Transfer RNA–guanine transglycosylase (Tgt, EC 2.4.2.29) catalyses the exchange of a specific guanine base in tRNA molecules by a substituted 7-deazaguanine. Bacterial Tgt functions as a homodimer in which the protomer consists of a (βα)8 barrel harbouring a Zn2+ binding subdomain close to the C-terminus. The reaction follows a ping-pong mechanism including a covalent Tgt⋅tRNA intermediate. Hence, in an attempt to generate a model system for the active site of human Tgt and to gain insights into the relevance of particular amino acids for substrate base selectivity, we adapted the Z. mobilis Tgt active site by site-directed mutagenesis in order to mimic that of the human enzyme.

Comparison of the active centre of Z. mobilis Tgt with the modelled human Tgt catalytic subunit reveals that Ala232 adjacent to Val233 in the bacterial enzyme is replaced by a serine (Ser231) in human Tgt. As this residue is replaced by a serine in many bacterial Tgts too, it seems unlikely that it contributes to substrate specificity or catalytic activity. Nevertheless, we introduced the Ala232Ser mutation into Tgt(Cys158Val/Val233Gly) to investigate its impact. Kinetic measurements showed that the Ala232Ser conversion further reduced the catalytic activity of Tgt(Cys158Val/Ala232Ser/Val233Gly). Therefore, the Ala232Ser variants of Tgt were not considered further in this study. In addition, crystal structures that were determined of Tgt(Cys158Val/Ala232Ser/Val233Gly) in its apo-form, in complex with preQ1 and in complex with queuine do not show any significant differences to the corresponding ones of Tgt(Cys158Val/Val233Gly) and, due to redundance, will not be discussed in detail (data statistics and PDB codes of these structures are provided in Table S2 of the Supporting Information).

> VEATAQETDRPRFSFSIAAREGKARTGTIEMKRGVIRTPAFMPVGTAATVKALKPETVRATGADIILGNTYHLMLRPGAERIAKLGGLHSFMGWDRPILTDSGGFQVMSLSSLTKQSEEGVTFKSHLDGSRHMLSPERSIEIQHLLGSDIVMAFDEVTPYPATPSRAASSMERSMRWAKRSRDAFDSRKEQAENAALFGIQQGSVFENLRQQSADALAEIGFDGYAVGGLSGGEGQDEMFRVLDFSVPMLPDDKPHYLMGVGKPDDIVGAVERGIDMFDCVLPTRSGRNGQAFTWDGPINIRNARFSEDLKPLDSECHCAVCQKWSRAYIHHLIRAGEILGAMLMTEHNIAFYQQLMQKIRDSISEGRFSQFAQDFRARYFARNS> MGHHHHHHQQLASFLSGTWQSGRGRSRLIHHAISGEALWEVTSEGLDMAAARQFAIEKGAPALRAMTFIERAAMLKAVAKHLLSEKERFYALSAQTGATRADSWVDIEGGIGTLFTYASLGSRELPDDTLWPEDELIPLSKEGGFAARHLLTSKSGVAVHINAFNFPCWGMLEKLAPTWLGGMPAIIKPATATAQLTQAMVKSIVDSGLVPEGAISLICGSAGDLLDHLDSQDVVTFTGSAATGQMLRVQPNIVAKSIPFTMEADSLNCCVLGEDVTPDQPEFALFIREVVREMTTKAGQKCTAIRRIIVPQALVNAVSDALVARLQKVVVGDPAQEGVKMGALVNAEQRADVQEKVNILLAAGCEIRLGGQADLSAAGAFFPPTLLYCPQPDETPAVHATEAFGPVATLMPAQNQRHALQLACAGGGSLAGTLVTADPQIARQFIADAARTHGRIQILNEESAKESTGHGSPLPQLVHGGPGRAGGGEELGGLRAVKHYMQRTAVQGSPTMLAAISKQWVRGAKVEEDRIHPFRKYFEELQPGDSLLTPRRTMTEADIVNFACLSGDHFYAHMDKIAAAESIFGERVVHGYFVLSAAAGLFVDAGVGPVIANYGLESLRFIEPVKPGDTIQVRLTCKRKTLKKQRSAEEKPTGVVEWAVEVFNQHQTPVALYSILTLVARQHGDFVD

To investigate the performance of the microscope in practical biological structure determination, we chose eleven macromolecular specimens with different sizes and symmetries to show that the capabilities of the instrument span the full range of molecular structures for which the single-particle cryoEM method is ideally suited. We determined eleven structures, with three having four identical molecular subunits, three having twelve identical subunits, and one structure each having 1, 5, 6, 24, and 60 subunits. When compared to the range of atomic structures determined by cryoEM in the PDB in recent years, we can therefore conclude that the system overall works well for nearly all specimens amenable to single-particle cryoEM. It is notable that all the structures were obtained with a single day of data collection where the number of one megapixel images in each case was between 350 and 500, equivalent to 20-30 images from the current generation of 16-megapixel direct electron detectors in use at 300 keV. The resolutions were all sufficient to build accurate atomic models (2.6–4.5 Å), and a majority of the structures (7 of 11) extended to beyond physical Nyquist resolution, indicating the power and importance of combined detector and optical performance.

Two of the others were essentially at Nyquist resolution (catalase and glutamine synthetase at 3.4 Å), with only PaaZ and the 70S ribosome at 0.9 Nyquist.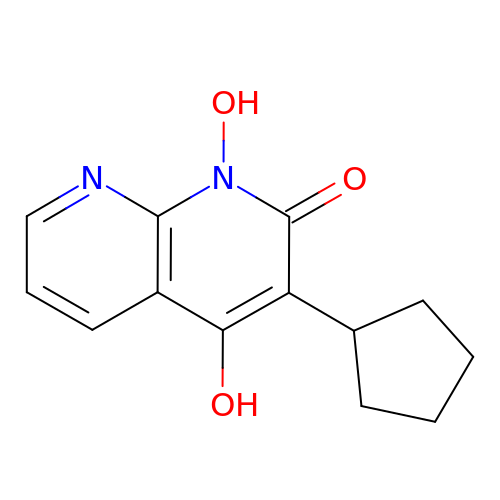3-cyclopentyl-1,4-dihydroxy-1,8-naphthyridin-2(1H)-one | C13 H14 N2 O3 | QHMJHXXRZXAFLA-UHFFFAOYSA-N> MDSCHKIDYGLYALEILAQYHNVSVNPEEIKHRFDTDGTGLGLTSWLLAAKSLELKVKQVKKTIDRLNFISLPALVWREDGRHFILTKVSKEANRYLIFDLEQRNPRVLEQSEFEALYQGHIILIASRSSVTGKLAKFDFTWFIPAIIKYRKIFIETLVVSVFLQLFALITPLFFQVVMDKVLVHRGFSTLNVITVALSVVVVFEIILSGLRTYIFAHSTSRIDVELGAKLFRHLLALPISYFESRRVGDTVARVRELDQIRNFLTGQALTSVLDLLFSFIFFAVMWYYSPKLTLVILFSLPCYAAWSVFISPILRRRLDDKFSRNADNQSFLVESVTAINTIKAMAVSPQMTNIWDKQLAGYVAAGFKVTVLATIGQQGIQLIQKTVMIINLWLGAHLVISGDLSIGQLIAFNMLAGQIVAPVIRLAQIWQDFQQVGISVTRLGDVLNSPTESYHGKLALPEINGNITFRNIRFRYKPDSPVILDNINLSIKQGEVIGIVGRSG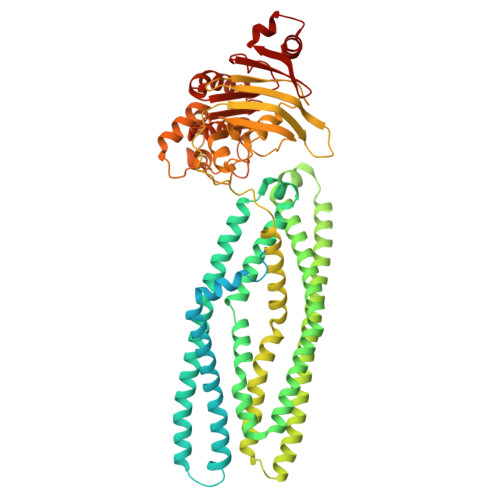SGKSTLTKLIQRFYIPENGQVLIDGHDLALADPNWLRRQVGVVLQDNVLLNRSIIDNISLANPGMSVEKVIYAAKLAGAHDFISELREGYNTIVGEQGAGLSGGQRQRIAIARALVNNPKILIFDEATSALDYESEHIIMRNMHKICKGRTVIIIAHRLSTVKNADRIIVMEKGKIVEQGKHKELLSEPESLYSYLYQLQSD> MPRPRVLLLGDPARHLDDLWSDFQQKFEVIPANLTTHDGFKQALREKRYGDFEAII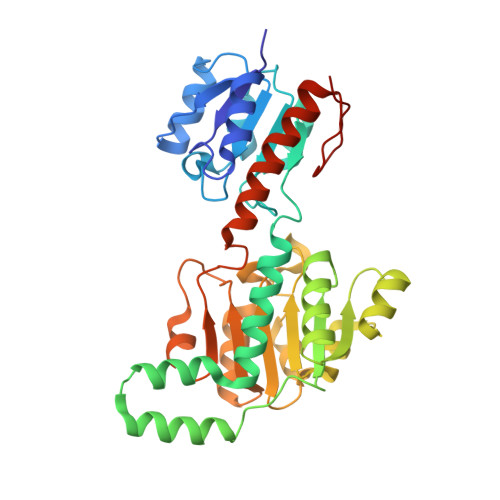KLAVENGTESYPWNADLISHLPSSLKVFAAAGAGFDWLDLDALNERGVAFANSRGAGDTATSDLALYLILSVFRLASYSERAARTGDPETFNRVHLEIGKSAHNPRGHVLGAVGLGAIQKEIARKAVHGLGMKLVYYDVAPADAETEKALGAERVDSLEELARRSDCVSVSVPYMKLTHHLIDEAFFAAMKPGSRIVNTARGPVISQDALIAALKSGKLLSAGLDVHEFEPNVSKELIEMKHVTLTTHIGGVAIETFHEFERLTMTNIDRFLLQGKPLLTPAGKVFAPSSAA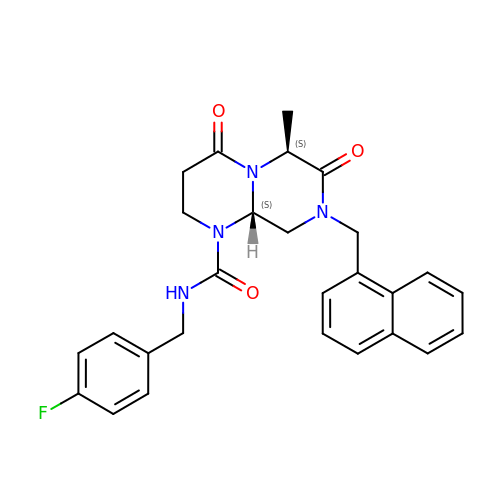(5S,6S,9aS)-N-[(4-fluorophenyl)methyl]-6-methyl-8-[(naphthalen-1-yl)methyl]-4,7-dioxohexahydro-2H-pyrazino[1,2-a]pyrimidine-1(6H)-carboxamide | C27 H27 F N4 O3 | UJSSMRPTIGCTEH-MHECFPHRSA-N>[6x]MPKPYVAINMAELKNEPKTFEMFASVGPKVCMVTARHPGFVGFQNHIQIGILPFGNRYGGAKMDMTKESSTVRVLQYTFWKDWKDHEEMHRQNWSYLFRLCYSCASQMIWGPWEPIYEIIYANMPINTEMTDFTAVVGK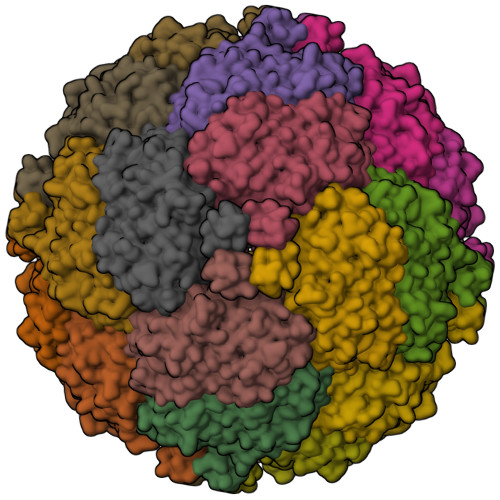KFAEGKPLDIPVISQPYGKRVVAFAEHSVIPGKEKQFEDAIVRTLEMLKKAPGFLGAMVLKEIGVSGIGSMQFGAKGFHQVLENPGSLEPDPNNVMYSVPEAKNTPQQYIVHVEWANTDALMFGMGRVLLYPELRQVHDEVLDTLVYGPYIRILNPMMEGTFWREYLNENAWRHPQFGG Ricin is a heterodimeric ribosome-inactivating protein (RIP) that is available worldwide in ton quantities as a byproduct of castor-oil production from the plant Ricinus communis. RTA is an efficient N-glycosidase that catalyzes the hydrolysis of a specific adenine within the 28S rRNA of the 60S ribosomal subunit, leading to cell death. RiVax is a recombinant protein that is currently under clinical development as part of a human vaccine to protect against ricin poisoning. RiVax includes ricin A-chain (RTA) residues 1–267 with two intentional amino-acid substitutions, V76M and Y80A, aimed at reducing toxicity.

The RiVax immunogen is a double mutant of RTA that combines the Y80A mutation to inactivate catalysis with the V76M mutation to ensure the removal of any trace VLS activity from the immunogen. Here, the crystal structure of RiVax was solved to 2.1 Å resolution and it was shown that it is superposable with that of the ricin toxin A-chain from Ricinus communis with a root-mean-square deviation of 0.6 Å over 258 Cα atoms. The X-ray crystal structure can be superposed onto that of RTA with a root-mean-square deviation (r.m.s.d.) of 0.6 Å over 258 Cα atoms, demonstrating that the Y80A and V76M mutations found in RiVax do not significantly perturb the overall protein fold or alter the conformation of residues corresponding to known neutralizing epitopes. Neither the active-site mutation (Y80A) nor the VLS mutation (V76M) significantly alters the side-chain conformations of adjacent residues. The enzymatic activity of RTA is the primary source of toxicity and therefore must be attenuated for safe vaccine development; this can be achieved by the introduction of a single point mutation, Y80A. Disruption of the VLP by a V76M mutation was shown to prevent RTA-induced weight loss, a biological marker of VLS, in specific animal models. The HTH contains a type I reverse turn between Phe181 and Ile184 which connects the two antiparallel helices of RiVax. In contrast to RiVax or RTA, the crystal structure of the RTA 1–33/44–198 R48C/T77C immunogen reveals that truncation of the C-terminus converts the HTH into a helical segment. Examination of the GD-12 epitope in the X-­ray crystal structures suggests that unlike UNIVAX 70/138, the binding site for GD-12 is partially buried in the folded protein. The results demonstrate the composition of the RiVax clinical material and will guide ongoing protein-engineering strategies to develop improved immunogens.

> MIFPKQYPIINFTTAGATVQSYTNFIRAVRGRLTTGADVRHEIPVLPNRVGLPINQRFILVELSNHAELSVTLALDMTNAAVVGYRAGNSAYFFHPDNQEDAEAITHLFTDVQNRYTFAFGGNYDRLEQLAGNLRENIELGNGPLEEAISALYYYSTGGTQLPTLARSFIICIQMISEAARFQYIEGEMRTRIRYNRRSAPDPSVITLENSWGRLSTAIQESNQGAFASPIQLQRRNGSKFSVYDVSILIPIIALMVYRCAPPPSSQF Here, we analyzed the uptake of LNB and its fucosylated H1 and Lea trisaccharides, as well as the mucin-derived disaccharide galacto-N-biose (GNB; Galβ1,3GalNAc) by an ABC importer from the HMO-utilization specialist Bifidobacterium longum subsp. infantis. Specialized extracellular solute binding proteins (SBPs) associated with ABC transporters mediate high-affinity capture of ligands for translocation into the cytoplasm through permease domains. Based on these data, Blon_0883 from B. infantis is henceforth designated as a GNB and fucosylated LNB-binding protein (BiGFL-BP). BiGFL-BP adopts a canonical SBP fold (structural cluster B), comprising two domains joined by a tripartite hinge with the ligand binding site located at the domain interface.

The Lewis a (Lea) and blood group H type 1 antigen (H1) trisaccharides were both bound with about four-fold lower affinity than the preferred LNB ligand. To bring insight into the binding of fucosylated LNB forms, we attempted to co-crystallize BiGFL-BP with a commercial preparation of Leb, which resembles a superimposition of H1 and the Lea trisaccharides to assess whether the protein can accommodate both fucosylations simultaneously. Surprisingly, the structure of the co-crystallized BiGFL-BP, revealed electron density for the α-1,2-linked fucose (Fuc) to the Gal unit of LNB, that is, we got the structure of the protein in complex with the H1 trisaccharide. This indicates that binding to the Leb tetrasaccharide is too weak or unfeasible, relative to the H1 trisaccharide, which may have been a contaminant present in the commercial preparation. Interestingly, a partially solvent-accessible cavity large enough to accommodate a monosaccharide was observed facing the C2-OH of the Gal moiety, another less spacious cavity was observed at the region around the C4-OH of the GlcNAc in LNB. Potential hydrogen bonds from the side chain of T101 to the C3-OH and C4-OH of the fucosyl unit were observed, whereas the main chain amide of the same residue has a potential hydrogen bond to the C4-OH. Another hydrogen bond from T205 to the C2-OH of the fucosyl was observed. Notably, the methyl group of the fucosyl unit is accommodated by an apolar pocket formed mainly by the F44 and the Cα-Cβ bond of S100. The electron density of the fucosyl is less well-defined than that of the LNB backbone, indicating the potential flexibility of this sugar ring.

> MTHFSTVKRVIALAGAGAMLFSVAACGGVTASDGGKTTLKFAAFEGGYGADMYKEVVAAYEKLNPDVKIELTTSKKIEDEITPGMKAGNYPDIVELGQGSTSGLTETLLKDKAIEDVTDVLDMKVPGENKTVKDKLVDGVIGLYTNPYGGDKTYLMPMYYSPSGLVYNKTLLEQNGWKMPTTWDEMFKLGDEAKAKGISLFTYPTAGYFDAFFNALLADIGGDQFYQDVMTYKKDVWKTDEAKEALETTYKLVTEYLNPDTVGYANAQDFTKNQQSILDGKSLFMPNGTWIVNEMKDAPRTSGFEWGFAPVPTVKNGGTRYINTTIEAVWIPAKAKNKEAAKKFMAYLYSDEAASIFAKTGAIQPIKGNTDDLASDMKVFYDAYNEDNVKAVAGSFSATATVEGKNIKDDLYNAVDSVASGKTTLQQWQDKLNETSNALNAAAKQ> MSKQFVRSAKNLVKGYSSTQVLVRNATSNDNHQVSKDSLIELAEKSYDSADFFEIMDMLDKRLNDKGKYWRHIAKALTVIDYLIRFGSENCVLWCRENLYIIKTLKEFRHEDDEGIDQGQIVRVKAKELTALLSDDERLNEERNMNIKGRNRKG;> DSDLQKALKKACSVEETAPKRKHVRACIVYTWDHQSSKAVFTTLKTLPLANDEVQLFKMLIVLHKIIQEGHPSALAEAIRDRDWIRSLGRVHSGGSSYSKLIREYVRYLVLKLDFHAHHRGFNNGTFEYEEYVSLVSVSDPDEGYET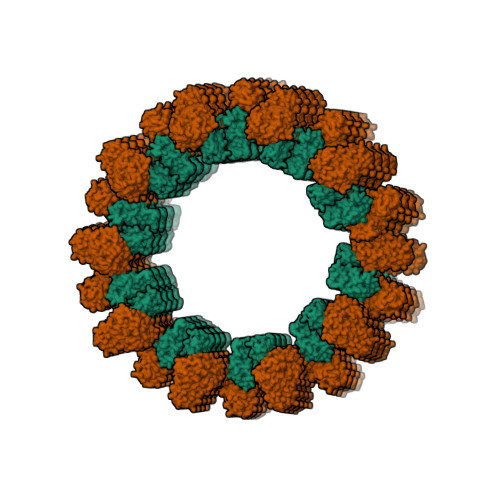ILDLMSLQDSLDEFSQIIFASIQSERRNTECKISALIPLIAESYGIYKFITSMLRAMHRQLNDAEGDAALQPLKERYELQHARLFEFYADCSSVKYLTTLVTIPKLPVDAPDVFLINDVDE Previous studies suggest mitochondrial ABCB7-type exporters are involved in maturation of cytosolic iron-sulfur proteins. Here, we report a series of cryo-electron microscopy structures of a eukaryotic homolog of human ABCB7, CtAtm1, determined at average resolutions ranging from 2.8 to 3.2 Å, complemented by functional characterization and molecular docking in silico. We propose that CtAtm1 accepts delivery from glutathione-complexed iron-sulfur clusters. As anticipated, the architecture of CtAtm1 harbors the classical ABC-fold, packing into a homodimer with six transmembrane segments (TM1–TM6) in each monomer.

Next, we determined a single particle cryo-EM structure at an average resolution of 3.0 Å, CtAtm1inw-opn, exploiting wild-type protein without supplementation of cargo but in the presence of ATP. The computed maps display well-resolved TM-domains, while the resolution of the NBDs is somewhat lower, and hence we are unable to confirm the absence of nucleotide binding. Nevertheless, de novo building of almost the entire structure was possible (580 modeled amino acids), with the exception of the first 94 residues in the N-terminus that includes the signal sequence for mitochondrial localization, and the last 26 residues of the C-terminus, likely related to flexibility of both termini. Thus, the configuration is distinct from the available structure of eukaryotic ScAtm1 and hABCB7 (PDB-ID 4MYC27, 7PSL28 and 7VGF26, RMSD 4.2, 3.8, and 3.2 Å), in which the NBDs interact via C-terminal extended helices in the S. cerevisiae structures. As such, our structure is more open, exposing a large cavity (>7000 Å3 as calculated using the software CastP3.0 with a 2.5 Å radius probe) that spans more than half of the membrane into the TM-domain. The cleft is decorated throughout with electropositive amino acids and is partially blocked at several levels: (1) at the matrix-membrane interface through the Asn395 pair of TM6 (one per monomer, conserved among eukaryotic Atm1), establishing an “inner” gate (the first from the mitochondrial matrix), and additional residue pairs closer toward the mitochondrial intermembrane space that firmly links the TM6 pairs. Notably, these amino acids also divide the cavity from Asn395 into two separate, symmetrically related, parts. We propose the inward-open configuration represents the resting state of eukaryotic Atm1 proteins, in which the protein exposes a highly electropositive cleft to the inside of the mitochondrial matrix, as detected in the CtAtm1inw-opn (and E603QCtAtm1inw-opn) structure.

>[2x]MSPRSRLLASSLRGGLLLRPCSARRSTLLNPSPSPLRKAIFHTTSLRAFKNLAEIATSSKEDASSLKPKGKPSPPGDPLATIEKTAAEQRRADWAIIKQMSRYLWPKDSWSDKARVLLALSLLVGGKVLNVHVPFYFREIIDRLNIDVAAVGGTVSAVAGAVIFAYGASRIGAVVSQELRNAVFSSVAQKAIRRVATQTFGHLLNLDLSFHLSKQTGGLTRAIDRGTKGISYLLTSMVFHIVPTALEIGMVCGILTYQFGWEFAAITAATMAAYTAFTITTTAWRTKFRRQANAADNAASTVAVDSLINYEAVKYFNNEAYEIARYDKALQAYERSSIKVATSLAFLNSGQNIIFSSALTLMMWLGARGVLAGDLSVGDLVLINQLVFQLSVPLNFLGSVYRELRQSLLDMETLFDLQKVNVTIREAPNAKPLALPKGGEIRFENVTFGYYPDRPILRNLSLTIPAGKKVAVVGPSGCGKSTLLRLLFRSYDPQQGKIFIDDQDIKSVTLESLRKSIGVVPQDTPLFNDTVELNIRYGNVNATQEQVIAAAQKAHIHEKIISWPHGYQTRVGERGLMISGGEKQRLAVSRLILKDPPLLFFDEATSALDTHTEQALMANINEVVKEKKRTALFVAHRLRTIYDADLIIVLKEGVVVEQGSHRELMERDGVYAELWMAQEMLHQGEAAEEPAEGEKAEEKK> MGGKWSKSSIVGWPAIRERLRRAQPAAERRRAQPAAEGVGAASQDLGRHGALTSSNTDTTNADEEEEVGFPVRPQVPLRPMTYKGAVDLSFFLKEKGGLEGLVYSQKRKEILDLWVYHTQGYFPDWQCYTPGPGVRYPLTFGWCFKLVPVDPGEVEEATEGENNC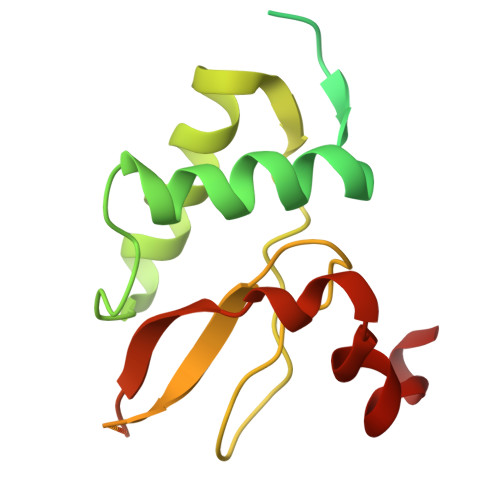LLHPICQHGMDDDHREVLKWKFDSHLAHTHMARELHPEFYKNC~{N}-[(2~{S})-1-[[(2~{R})-2,3-dimethylbutyl]amino]-4-methyl-1-oxidanylidene-pentan-2-yl]-(phenylmethoxycarbonylaminomethyl)phosphonamidic acid | C21 H36 N3 O5 P 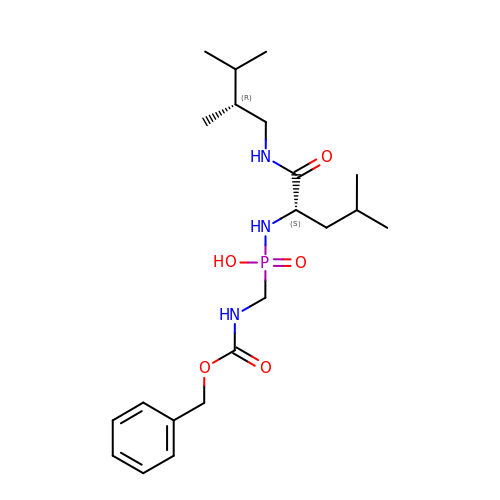| JBYBUNCIQMPTHL-HKUYNNGSSA-N> YLDLFSHKNMKLKE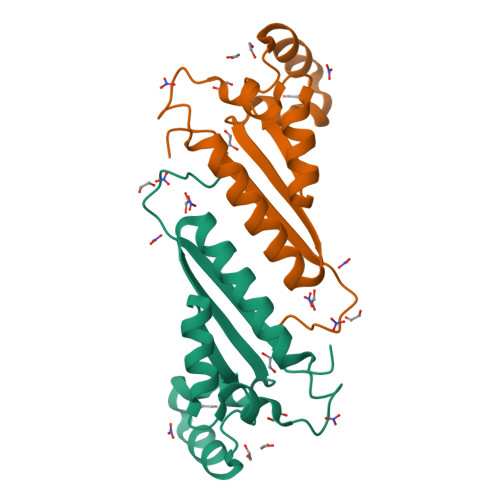RVLIPVKQYPKFNFVGKILGPQGNTIKRLQEETGAKISVLGKGSMRDKAKEEELRKGGDPKYAHLNMDLHVFIEVFGPPCEAYALMAHAMEEVKKFLVPDM>[2x]HMNYRELIERARRTTAAEEYDISGRYPSVIAHAEGAWMTDLSGNRYVDLTGADAAVILGYRHPAVNEAITRQIRDYGTTFASTLSVPRVELAERMCERYECAEKVVFHKTGTEGTAMAVRLARAATGRELVLSSGYHGWHEWQMAGEEFGYQQSTGVVGFGYNEKALAKMLEAFGEQVAGVIVSPEVLYFDLDHYRRMSALCARYDVPFMLDEVYTGFRAGPKGVHGLGVPADVVVLGKGLAN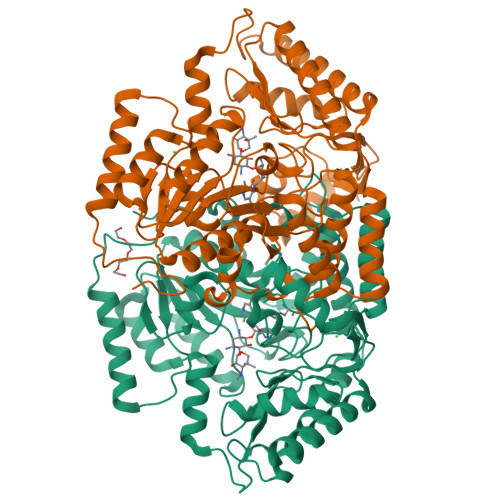GHSLAAVMGRRDIIDAYDVSGIQGTYTREVPPMAAALAVFEVLDTPGVYEHAEAMGRRLADGMREILTGEGIPNWVGGPALMFDVVLPNDDLGWEIYKTAHDFGVYFEDSGTQLVTAAFDEAAVDHALTAFRKATRQVVADRPDIAPTSGGELTEERKLDFAEEAFGGLLRDDERTNALIDETIEKVVNRDRSIKPVLFPAQN>[2x]GENSDNLTHCRLFEFRLCLLECMSLTLDHCYARCTTVITQIHGSDTNRFDCTIFKTCYYRCYVLGKTEDHCWKGTATSVTGDVGDLEFC

The venoms of marine cone snails constitute a particularly rich source of peptide toxins, known as conotoxins. Here, we identify the sequence of an unusually large conotoxin, Mu8.1, which defines a new class of conotoxins evolutionarily related to the well-known con-ikot-ikots and 2 additional conotoxin classes not previously described. The crystal structure of recombinant Mu8.1 displays a saposin-like fold and shows structural similarity with con-ikot-ikot. Functional studies demonstrate that Mu8.1 curtails calcium influx in defined classes of murine somatosensory dorsal root ganglion (DRG) neurons. When tested on a variety of recombinantly expressed voltage-gated ion channels, Mu8.1 displayed the highest potency against the R-type (Cav2.3) calcium channel.

To elucidate key structural features of the SLC superfamily, we determined crystal structures of Mu8.1 from 2 different crystal conditions referred to as Mu8.1_38 and 59 at resolutions of 2.33 Å and 2.1 Å, respectively. The asymmetric unit of Mu8.1_38 includes 2 molecules that form a single dimer with an interface equivalent to the one present in the 3 dimers in Mu8.1_59. Each protomer of the Mu8.1 structure comprises 2 regions. The first region comprises an N-terminal 310-helix (310N), followed by 2 α-helices (α1 and α2), and a 310-linker helix (310L). The second region comprises 2 α-helices (α3 and α4), and the C-terminal 310-helix (310C). The disulfide bonds are found primarily within each of these 2 regions. Within the first region, the Cys18-Cys34 and Cys22-Cys30 disulfide bonds connect α1 and α2. Further, the 310N-helix connects to α3 through the Cys10-Cys51 disulfide bond. In the second region, Cys61-Cys71 links α3 and α4, and Cys57-Cys89 tethers the C-terminus to α3. The dimer interface is characterized by both hydrophobicity as well as the presence of a water-filled cavity surrounded by the polar residues Thr36, Asn47, Thr52, and Thr56.>[2x]LGSS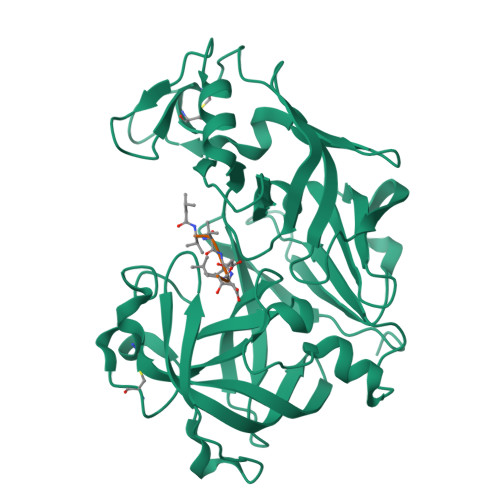NDNIELVDFQNIMFYGDAEVGDNQQPFTFILDTGSANLWVPSVKCTTAGCLTKHLYDSSKSRTYEKDGTKVEMNYVSGTVSGFFSKDLVTVGNLSLPYKFIEVIDTNGFEPTYTASTFDGILGLGWKDLSIGSVDPIVVELKNQNKIENALFTFYLPVHDKHTGFLTIGGIEERFYEGPLTYEKLNHDLYWQITLDAHVGNISLEKANCIVDSGTSAITVPTDFLNKMLQNLDVIKVPFLPFYVTLCNNSKLPTFEFTSENGKYTLEPEYYLQHIEDVGPGLCMLNIIGLDFPVPTFILGDPFMRKYFTVFDYDNHSVGIALAKKNL>[2x]DRH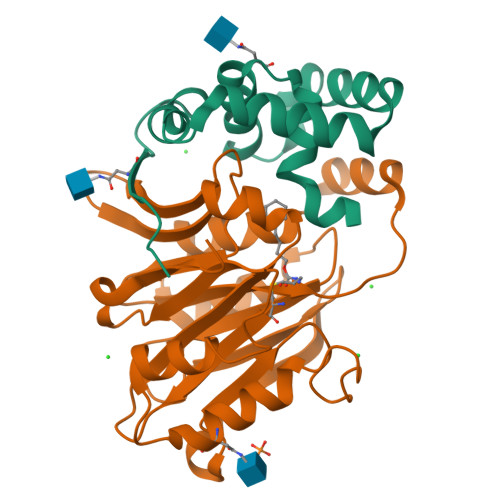HHHHHGSPAPPRVNVSLDAAPAARWLPVLRLFDPGLLRAAVARIVGDRVPKWVRDVIGKLVAEMESFLPQPYTEEIRGISDFLNLSLADGFIVNLAYEASAF;>[2x]CTSVVAQDSRGHIYHGRNLDYPFGDLLRKMTVDVQFLKNGQIAFTGTTFIGYVGLWTGQSPYKFTVSGDERADKGWWWENMIAALFQGHSPVSWLIRTTLSESEDFEASVYKLAKTPLIADVYYIVGGTAPGEGVVVTRNRGGPADIWPLDPLNGAWFRVETNYDHWKPVPKSDDRRTPAIKALNATGQANLSLEALFQVLSVVPVCNKITVYTTVMSAATPDKYMTRIRNLS> EDDDDKDQDESD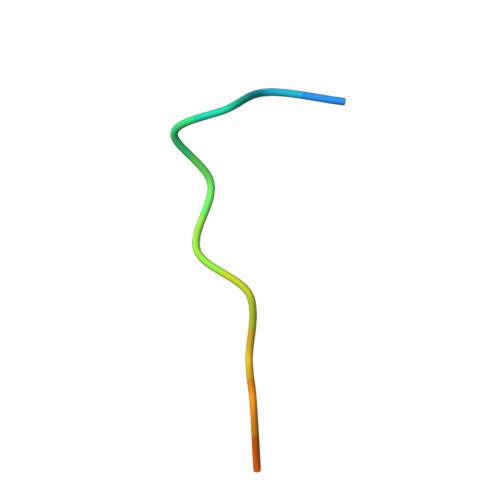SDT> GPGSVAEAPSYQGPPPPYPKHLLHQN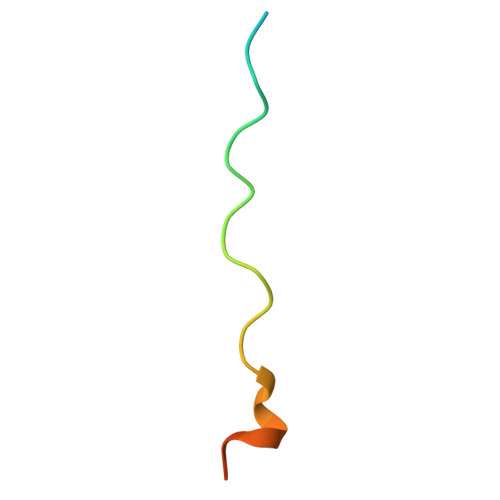PS>[2x]TEEKTCDLVGEKGKESEKQLALLKRLTPLFQKSFESTVGQSPDMYSYVFRVCREAGQHSSGAGLVQIQKSNGKETVVGRFNETQIFQGSNWIML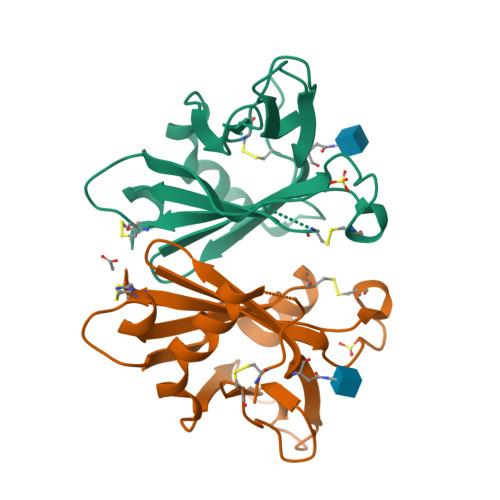IYKGGDEYDNHCGREQRRAVVMISCNRHTLADNFNPVSEERGMVQDCFYLFEMDSSLACS> GPLGSMEKTYGKTVLPLSRVKRIIK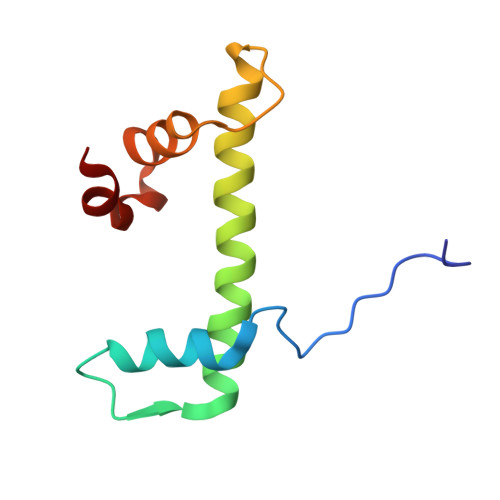QDEDVHYCSNASALLISVATELFVEKLATEAYQLAKLQKRKGIRYRDVEDVVRKDDQFEFLSDLFSI>[2x]MIFDKEDYKAFDPELWNAIDAEAERQQNNIELIASENVVS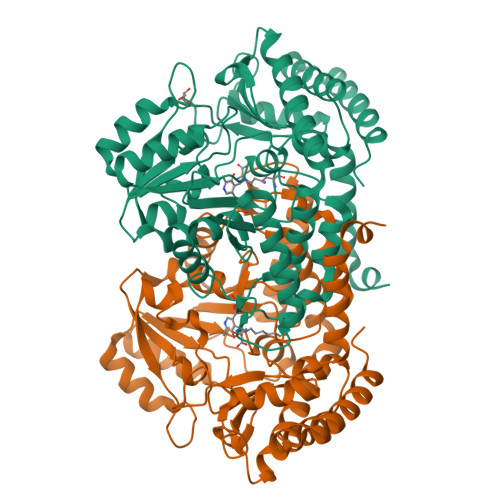KAVMAAQGTLLTNKSAEGYPGKRYYGGTAVIDVVETLAIERAKKLFGAKFANVQPHSGSQANAAVYMSLIQPGDTVMGMDLSAGGHLTHGAPVSFSGKTYNFVSYNVDKESELLDYDAILAQAKEVRPKLIVAGASAYSRIIDFAKFREIADAVGAYLMVDMAHIAGLVASGHHPSPVPYAHVTTTTTHKTLRGPRGGLILTDDEDIAKKLNSAVFPGLQGGPLEHVIAAKAVALKEALDPAFKEYGENVIKNAAAMADVFNQHPDFRVISGGTNNHLFLVDVTKVVENGKVAQNVLEEVNITLNKNSIPYEQLSPFKTSGIRVGSPAITSRGMGEAESRQIAEWMVEALENHDKPEVLERIRGDVKVLTDAFPLY> MGYLCNDYGYEPNVDYPNASHAGLYDRSKQPYVDTAIGPKTTIQFDHVFIKSDFKTWLAHNQDEAILLIRLYELGLLLQGRSDSFLEFYNNTTY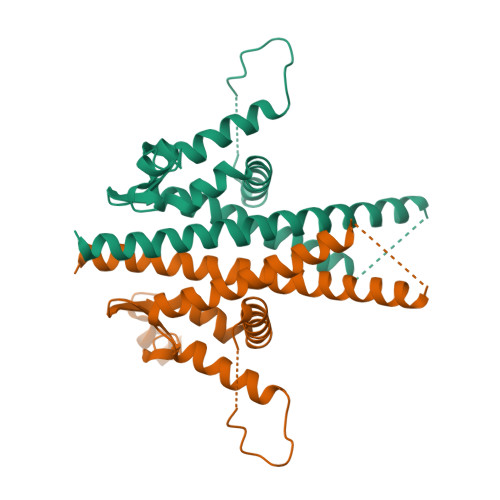ITRTDSKQPFLNKYGKLVDTTSVTCLDIFLSVVLFALNQIDSLICDFKNTPWINLSKEHKKIYELVRGIFGICYGEKDYNRFEYCPFDANSTASALNVNATLNAKKTIELITCGLIRALIAYANLVTAFSADKTALLHEILLTKVCC>MFVNLRNCVLGLLVAGATASPITKDLATIEKRQNLPNGVAIFKCTVPNTIALTFDDGPHIWTENAVNQLEAAGMKGTFFLNGKNFGELKNYVPLLKRMRANRHQIGSHTWDHPYLTQLSDAAVRKQMTDFENELRRLIGYYPTYMRPPYFDYNAKTLAVMKELGYRVIHADLDTNDWKFDMPASIAAFKAGVANNRIVLAHDVHETTVKTLLPAMIKEVQRLKLKAVTVGECLGEPYAYWYRVTPRAHHHHHH[5x]

Phytopathogenic fungi secrete chitin deacetylase (CDA) to escape the host’s immunological defense during infection. Five crystal structures of two representative and phylogenetically distant phytopathogenic fungal CDAs, VdPDA1 from Verticillium dahliae and Pst_13661 from Puccinia striiformis f. sp. tritici, were obtained in ligand-free and inhibitor-bound forms. These structures suggested that both CDAs have an identical substrate-binding pocket and an Asp-His-His triad for coordinating a transition metal ion. Our findings revealed that phytopathogenic fungal CDAs share common structural features, and provided BHA as a lead compound for the design of CDA inhibitors aimed at attenuating crop fungal diseases.

Gao et al. showed that the cotton root pathogen Verticillium dahliae secretes a CDA (VdPDA1) that is specifically localized to fungus-host interfaces. VdPDA1 prevents CO-induced immune response reactive oxygen species (ROS) production, MAPK phosphorylation, and resistance-related gene expression. VdPDA1 and Pst_13661 are single-domain enzymes with 55% sequence similarity. The substrate-binding grooves of VdPDA1 and Pst_13661 are short and open-ended. Both enzymes adopt a classic (β/α)7 fold. In the structure of VdPDA1, the signature Asp-His-His triad (formed by Asp56, His108 and His112) and a water molecule were coordinate with a metal ion. Kinetic studies also indicated that both VdPDA1 and Pst_13661 used the Zn2+ ion instead of the Ni2+ ion for their higher activity. The mutant VdPDA1D55A, H201A, which completely lost its deacetylase activity, was constructed. Using VdPDA1 as a model, we showed that the catalytic residue-mutated strain VdΔpda1/cPDA1D55A, H201A could not evade host plant defenses, suggesting that the deacetylase activity of fungal CDAs is crucial for full virulence.> MLSYFQGFVPIHTIFYSVFHPTEGSKIKYEFPPNNLKNHGINFNTFKNYIIPKPILCHKLITFKYGTYRIVCYPVTINSPIYARNFFSFNFVFVFPYDCETSPYEPAITRLGKMFKVLEEQNQLLSKSERDPVFFDLKVLENSTTTPSTAGPSSTPNPSSNTTPTHPTSEKDTKDMRSSRYSDLIKDLGLPQSAFSIQDLLMRIFQDLNNYSECLIPIDEGNAVDIKIFPLLRPPTTCVSLEDVPLSSVNLKKIIDVNWDPTMMSIVPYIDGLNSIAKIS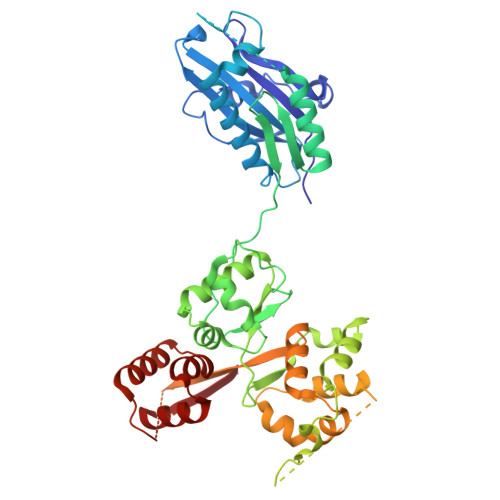KLSNSDPGLVIECIRHLIYYKCVTLSDIFQFSNIYAPSSLIRNFLTDPLMASDCQSYVTFPEVSKISNLPLNKSLGSGDQDSPSFSVRRKSKSSSIPSNPDSRTTSFSSTSRVSQNSSLNSSFSSIYKDWRQSQTSCSSSNIHVINNRNRFLPTRSCLFDLYRSLSQGQTLKTWYESKYMILKENNIDIRRFITFGLEKRIIYRCYSFPVMINAGSREPKEMTPIITKDLVNNDKLLEKRNHNHLLSATGSRNTAQSGNLKPERPSKVSFEMQRVSSLATGKSTMPKLSDEEEGILEESIRNAETFDKICVLLSKPKLEVESYLNELGEFKVINS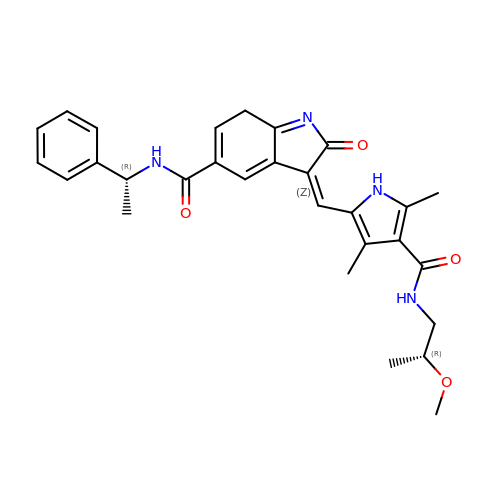(3Z)-3-[(4-{[(2R)-2-methoxypropyl]carbamoyl}-3,5-dimethyl-1H-pyrrol-2-yl)methylidene]-2-oxo-N-[(1R)-1-phenylethyl]-3,7-dihydro-2H-indole-5-carboxamide | C29 H32 N4 O4 | KCTMKOYMOWPPFA-ZNAXHXMPSA-N> SHMSRKIRDLIESKRFQNVITAIIVLNGAVLGLLTDTTLSASSQNLLERVDQLCLTIFIVEISLKIYAYGVRGFFRSGWNLFDFVIVAIALMPAQGSLSVLRTFRIFRVMRLVSVIPTMRRVVQGMLLALPGVGSVAALLTVVFYIAAVMATNLYGATFPEWFGDLSKSLYTLFQVMTLESWSMGIVRPVMNVHPNAWVFFIPFIMLTTLTVLNLFIGIIVDAMAITKEQEEEAKTGHHQEPISQTLLHLGDRLDRIEKQLAQNNELLQRQQPQKK

Voltage-gated sodium channels (Navs) specifically enable the passage of sodium ions across cell membranes, contributing to the electrical signalling in cells. Mutations in hNavs have been associated with a range of channelopathies, including pain, epilepsy, and heart disorders, making them major targets for drug development. The NavMs channel has been shown to be an excellent exemplar for hNavs as it exhibits highly similar functional, conductance, and drug-binding (similar IC50 values) characteristics, as well as sequence and structural homologies.

The compelling reason for using crystal structures of NavMs in this study is that they provide the, to date, highest resolution (~2.2–2.5 Å) views of any sodium channel, especially of the TM and drug-binding regions, thus enabling detailed views of the protein molecular structures with drugs bound to them. It should be noted here, that this region of the apo structure also exhibits some electron density (but has a different size and shape), which has been attributed to detergent molecules.> WSHPQFEKGA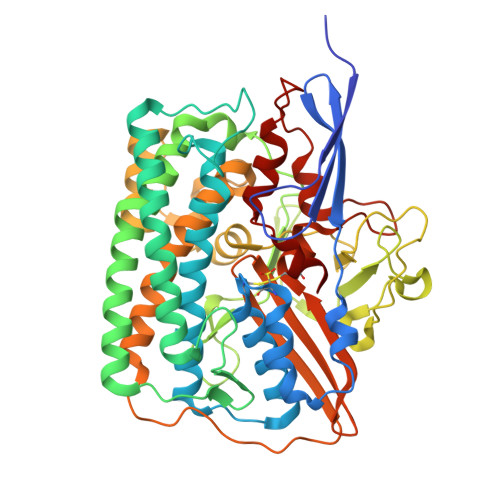TGRTTIAIDPVTRIEGHLKAEVVVENGKVVDARLSGTMYRGFETILRGRDPRDASQIVQRICGVCPTAHSTASVLALDEAFGAKVPNNGRITRNLIFGANYLQSHILHFYHLSAQDFVQGPDTAPFVPRFPKSDLRLSKELNKAGVDQYIEALEVRRICHEMVALFGGRMPHVQGQVVGGATEIPTKEKLVEYAARFKKVRDFVEQKYVPVVYTIGSKYKDMFKVGQGFKAALCVGAFPLDNSGKKHLFMPGVYAKGKDMPFDPSKIKEYVKYSWFAEETTGLNYKEGKTIPAPDKAGAYSFVKAPRYDGLSLEVGPLARMWVNNPELSPVGKKLLKDLFGISAKKFRDLGEEAAFSLMGRHVARAEETYYMLGAIEGWLKEIKAGEDTVVMPAVPASAEGTGFTEAPRGSLLHYVKVKDSKIDNYQIVSASLWNCNPRDDMGQRGAVEEALIGIPVDDIQNPVNVARLIRAFDPULGCAVH2-{[(E)-{3-hydroxy-2-methyl-5-[(phosphonooxy)methyl]pyridin-4-yl}methylidene]amino}prop-2-enoic acid | C11 H13 N2 O7 P | 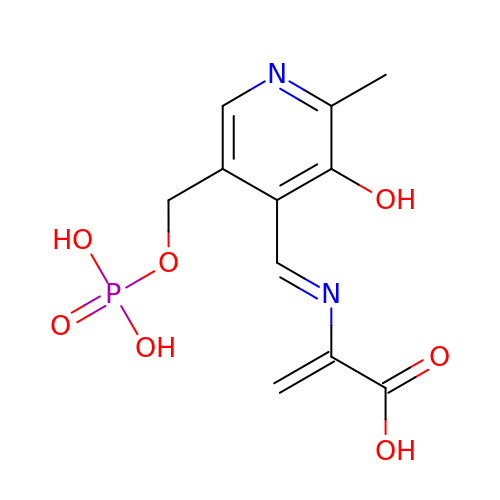BHIGINKEEFZJGX-YIXHJXPBSA-N>GSSHHHHHHSSGENLYFQGHMTCPFADPAALYSRQDTTSGQSPLAAYEVDDST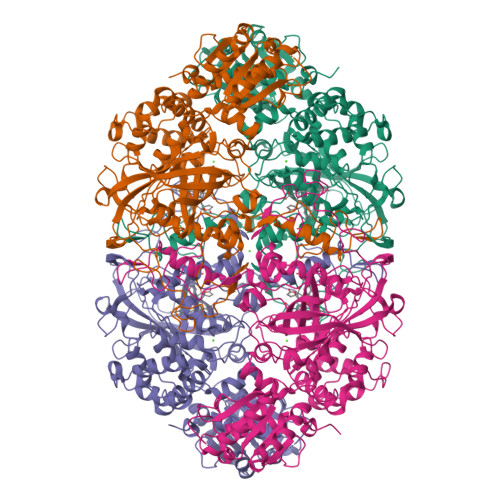GYLTSDVGGPIQDQTSLKAGIRGPTLLEDFMFRQKIQHFDHERVPERAVHARGAGAHGTFTSYADWSNITAASFLNATGKQTPVFVRFSTFAGSRGSADTARDVHGFATRFYTDEGNFDIVGNNIPVFFIQDAIQFPDLIHSVKPRPDNEIPQAATAHDSAWDFFSQQPSTMHTLFWAMSGHGIPRSYRHMDGFGVHTFRFVKDDGSSKLIKWHFKSRQGKASLVWEEAQVLSGKNADFHRQDLWDAIESGNGPEWDVCVQIVDESQAQAFGFDLLDPTKIIPEEYAPLTKLGLLKLDRNPTNYFAETEQVMFQPGHIVRGIDFTEDPLLQGRLFSYLDTQLNRNGGPNFEQLPINMPRVPIHNNNRDGAGQMFIHRNKYPYTPNTLNSGYPRQANQNAGRGFFTAPGRTASGALVREVSPTFNDHWSQPRLFFNSLTPVEQQFLVNAMRFEISLVKSEEVKKNVLTQLNRVSHDVAVRVAAAIGLGAPDADDTYYHNNKTAGVSIVGSGPLPTIKTLRVGILATTSESSALDQAAQLRTRLEKDGLVVTVVAETLREGVDQTYSTADATGFDGVVVVDGAAALFASTASSPLFPTGRPLQIFVDAYRWGKPVGVCGGKSSEVLDAADVPEDGDGVYSEESVDMFVEEFEKGLATFRFTDRFALDS[8x]> MAELRVLVAVKRVIDYAVKIRVKPDRTGVVTDGVKHSMNPFCEIAVEEAVRLKEKKLVKEVIAVSCGPAQCQETIRTALAMGADRGIHVEVPPAEAERLGPLQVARVLAKLAEKEKVDLVLLGKQAIDDDCNQTGQMTAGFLDWPQGTFASQVTLEGDKLKVERAIDGGLETLRLKLPAVVTADLRLNEPRYATLPNIMKAKKKKIEVIKPGDLGVDLTSKLSVISVEDPPQRTAGVKVETTEDLV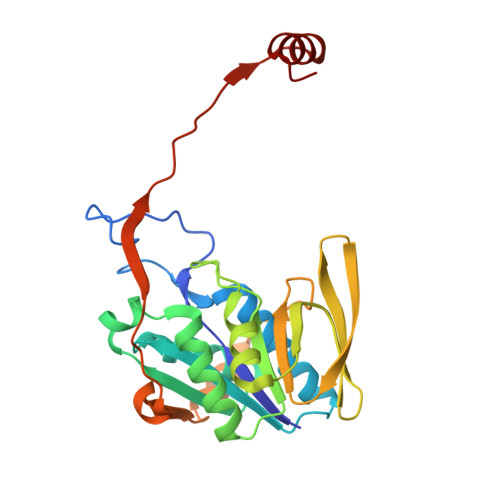AKLKEIGRI> PHMSGLKKFFPYSTNVLKGAAADIALPSLAGKTVFFYFSAS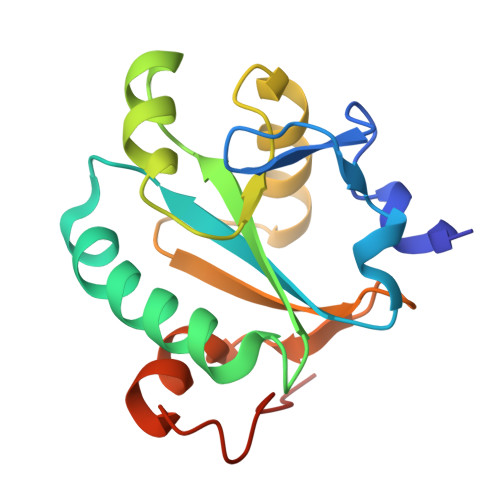WCPPCRAFTPQLIDFYKAHAEKKNFEVMLISWDESAEDFKDYYAKMPWLALPFEDRKGMEFLTTGFDVKSIPTLVGVEADSGNIITTQARTMVVKDPEAKDFPWPNVEAKK>[3x]SNA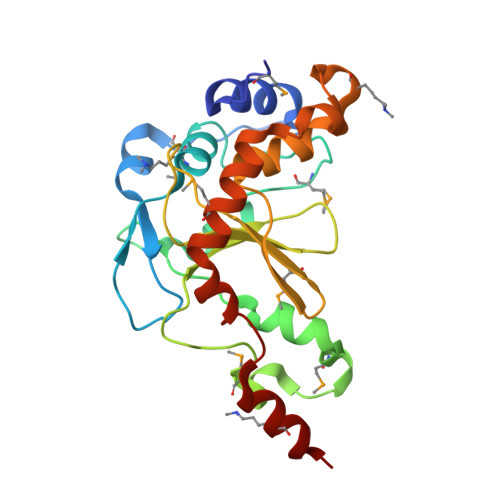MDISLTNLIELVKKVNRNKVPTPMSAEEISRLRVRKYRDPQNTETTELPESLKALLAYDRDLLSNYNMPVIETLQKSIDNEGVIHSYSPDEEAYYGVGMDSSGIDIEDLMPVWSNDPRLPALIRIDHVGDQAIFIYITERDANGEYPIARMERNEFWLAESSLVEYLYNIISGAKDIGFTEEDLHLPQWKAQQKMNEQRDAALLDLEDYHEAFWAKLDALVD>[4x]MGSDKIHHHHHHMVDDIFERGSKGSSDFFTGNVWVKMLVTDENGVFNTQVYDVVFE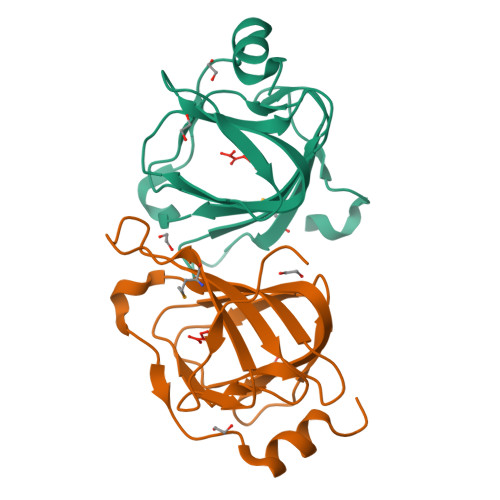PGARTHWHSHPGGQILIVTRGKGFYQERGKPARILKKGDVVEIPPNVVHWHGAAPDEELVHIGISTQVHLGPAEWLGSVTEEEYRKATEGK> DICRLCLRGVSGAQMCLQI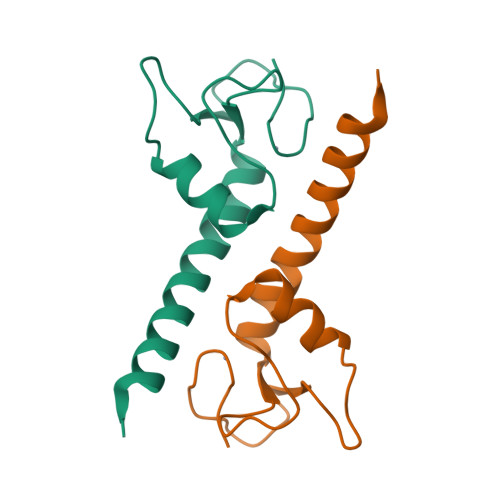FDVDSGESKVAEVLRQHFWFEVLPNDEISKVICNVCWTQVSEFHQFYVSIQEAQVIYATTS> MFVNKQFNYKDPVNGVDIAYIKIPNAGQMQPVKAFKIHNKIWVIPERDTFTNPEEGDLNPPPEAKQVPVSYYDSTYLSTDNEKDNYLKGVTKLFERIYSTDLGRMLLTSIVRGIPFWGGSTIDTELKVIDTNCINVIQPDGSYRSEELNLVIIGPSADIIQFECKSFGHDVLNLTRNGYGSTQYIRFSPDFTFGFEESL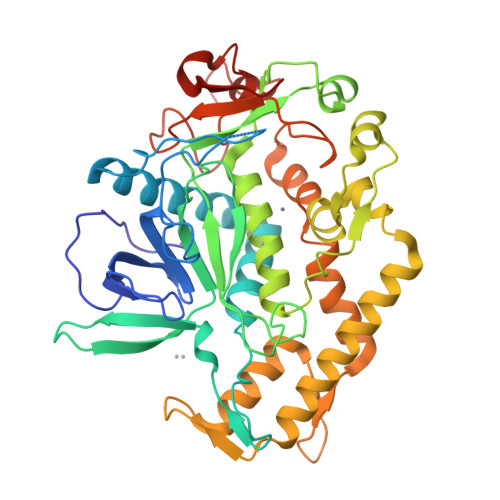EVDTNPLLGAGKFATDPAVTLAHELIHAEHRLYGIAINPNRVFKVNTNAYYEMSGLEVSFEELRTFGGHDAKFIDSLQENEFRLYYYNKFKDVASTLNKAKSIIGTTASLQYMKNVFKEKYLLSEDTSGKFSVDKLKFDKLYKMLTEIYTEDNFVNFFKVINRKTYLNFDKAVFRINIVPDENYTIKDGFNLKGANLSTNFNGQNTEINSRNFTRLKNFTGLFEFY> GPHMPGSGQIQLWQFLLELLSDSSNSSCITWEGTNGEFKMTDPDEVARRWGERKSKPNMNYDKLSRALRYYYDKNIMTKVHGKRYAYKFDFHGIAQALQPHPPESSLYKYPSDLPYMGSYHAHPQKMN;> AELVRTDSPNFLCSVLPSHWRCNKTLPVAFKVVALGEVPDGTVVTVMAGNDENYSAELRNASAVMKNQVARFNDLRFVGRSGRGKSFTLTITVFTNPPQVATYHRAIKVTVDGPREPRRHRQKLDDSKPSLFSDRLSDLGRIPHPSMRVGVPPQNPRPSLNSAPSPFNPQGQSQITD;> MGSSHHHHHHSQDPMPRVVPDQRSKFENEEFFRKLSRECEIKYTGFRDRPHEERQARFQNACRDGRSEIAFVATGTNLSLQFFPASWQGEQRQTPSREYVDLEREAGKVY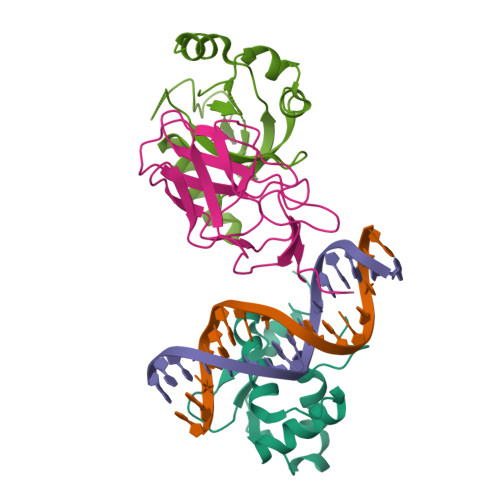LKAPMILNGVCVIWKGWIDLQRLDGMGCLEFDEERAQQEDALAQQA> ADERLQFTATTLSGAPFDGASLQGKPAVLWFWTPWCPFCNAEAP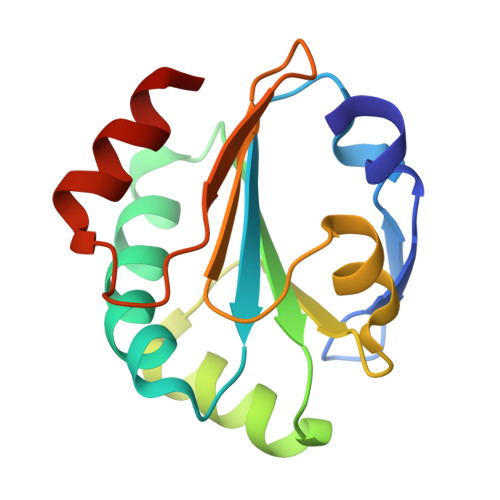SLSQVAAANPAVTFVGIATRADVGAMQSFVSKYNLNFTNLNDADGVIWARYNVPWQPAFVFYRADGTSTFVNNPTAAMSQDELSGRVAALTS> LADHPGELVRTDSPNFLCSVLPTHWRCNKTLPIAFKVVALGDVPDGTLVTVMAGNDENYSAELRNATAAMKNQVARFNDLRFVGRSGRGKS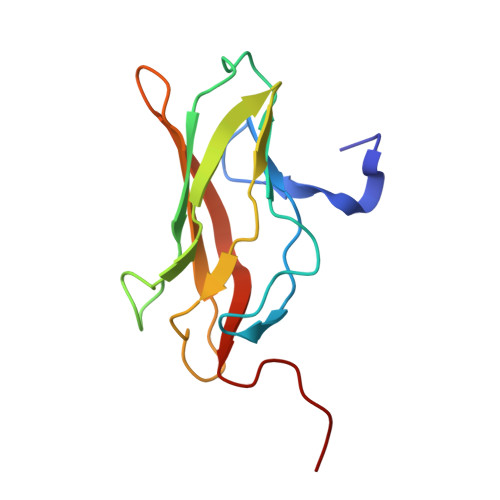FTLTITVFTNPPQVATYHRAIKITVDGPREPR>MSRNNDINAEVVSVSPNKLKISVDDLEEFKIAEEKLGVGSYLRVSDNQDVALLAIIDNFSIEVKESQKQKYMIEASPIGLVKNGKFYRGGDSLALPPKKVEPAKLDEIISIYSDSIDINDRFTFSSLSLNTKVSVPVNGNRFFNKHIAIVGSTGSGKSHTVAKILQKAVDEKQEGYKGLNNSHIIIFDIHSEYENAFPNSNVLNVDTLTLPYWLLNGDELEELFLDTEANDHNQRNVFRQAITLNKKIHFQGDPATKEIISFHSPYYFDINEVINYINNRNNERKNKDNEHIWSDEEGNFKFDNENAHRLFKENVTPDGSSAGALNGKLLNFVDRLQSKIFDKRLDFILGEGSKSVTFKETLETLISYGKDKSNITILDVSGVPFEVLSICVSLISRLIFEFGYHSKKIKRKSNENQDIPILIVYEEAHKYAPKSDLSKYRTSKEAIERIAKEGRKYGVTLLLASQRPSEISETIFSQCNTFISMRLTNPDDQNYVKRLLPDTVGDITNLLPSLKEGEALIMGDSISIPSIVKIEKCTIPPSSIDIKYLDEWRKEWVDSEFDKIIEQWSKS[6x];>MDRSAVDTIRGYCYQVDKTIIEIFSLPQMDDSIDIECIEDVDVYNDGHLTAIQCKYYESTDYNHSVISKPIRLMLSHFKDNKEKGANYYLYGHYKSGQEKLTLPLKVDFFKSNFLTYTEKKIKHEYHIENGLTEEDLQAFLDRLVININAKSFDDQKKETIQIIKNHFQCEDYEAEHYLYSNAFRKTYDISCNKKDRRIKKSDFVESINKSKVLFNIWFYQYEGRKEYLRKLKESFIRRSVNTSPYARFFILEFQDKTDIKTVKDCIYKIQSNWSNLSKRTDRPYSPFLLFHGTSDANLYELKNQLFNEDLIFTDGYPFKGSVFTPKMLIEGFSNKEIHFQFINDIDDFNETLNSINIRKEVYQFYTENCLDIPSQLPQVNIQVKDFADIKEIV[12x]

Here, we biochemically and structurally characterize a two-component defense system DUF4297–HerA, demonstrating that DUF4297–HerA confers resistance against phage infection by cooperatively cleaving dsDNA and hydrolyzing ATP. DUF4297 encodes a protein containing an N-terminal DUF4297 domain (a putative PD-(D/E)xK-family nuclease) with predicted yet-to-be biochemically characterized nuclease activity and a C-terminal domain (CTD) with unknown function. HerA, widely distributed in archaea and bacteria, encodes a DNA motor protein, which can hydrolyze ATP and translocate along DNA. The enzymatic activities and anti-phage defense function of the DUF4297–HerA system are activated through supramolecular assembly.

To reveal the assembly mode of this complex, we further determined the cryo-EM structure of DUF4297–HerA complex at an overall resolution of 2.87 Å with C2 symmetry imposed. The high quality of the cryo-EM density map allowed us to build the CTD of DUF4297, whereas only a partial part of the N-terminal DUF4297 domain was modeled due to the weak density of this region. The cryo-EM structure reveals that twelve DUF4297 molecules and six HerA molecules form a giant assembly with a molecular weight of ~1 MDa. The architecture of the resolved complex has a shape that resembles a human head in a hat, with a 172 Å × 172 Å × 180 Å dimension. The HerA forming a planar hexameric ring resembles the head, while twelve DUF4297 molecules, organized into the upper and the lower layers, resemble the hat. HerA forms a planar hexameric structure with a central pore in the DUF4297–HerA complex, which is significantly different from the nonplanar conformation of HerA alone. The base of the hexamer, supposed to be the DNA entry site, is closed by the insertion subdomain. The HAS domains and two layers of DUF4297 adopt a nearly C6 symmetric conformation with a continuous channel. Six DUF4297 molecules from the upper layer are held together primarily through mixed salt-bridge and hydrogen-bond interactions mediated by the adjacent CTD domains. Six DUF4297 molecules from the lower layer do not contact each other but form a tail-to-tail dimer with one neighboring DUF4297 from the upper layer through a loop connecting helices α3 and α4. The loops connecting helix α1 and β-strand β1, and helix α2 and β-strand β2 of CTD of the lower layer DUF4297 form extensive polar interactions with the HAS domain from HerA.>MGAQETIVIGLAADSGCGKSTFMRRLTSVFGGAAKPPKGGNPDSNTLISDTTTVICLDDYHSLDRYGRKEQKVTALDPRANDFDLMYEQVKALKNGIAVEKPIYNHVTGLLDPPELIQPPKILVIEGLHPMFDERVRDLLDFSIYLDISNEVKFAWKIQRDMAERGHSLESIKASIEARKPDFDA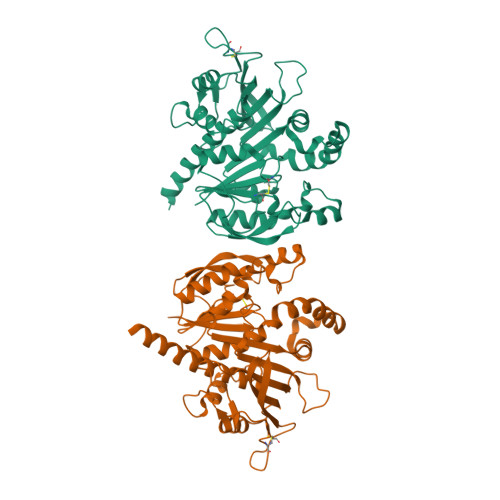FIDPQKQYADAVIEVLPTTLIPDDNEGKVLRVRLIMKEGVKYFSPVYLFDEGSTISWIPCGRKLTCSYPGIKFNYEPDSYFDHEVSVLEMDGQFDRLDELIYVESHLSNLSTKFYGEVTQQMLKHADFPGSNNGTGLFQTIVGLKIRDLYEQLIANKATARAEAKALEHHHHHH[2x]> SRVLLALHDRAPQLKISDDRLTVVGEKGYSMVRASHGVRKGAWYFEITVDEMPPDTAARLGWSQPLGNLQAPLGYDKFSYSWRSKKGTKFHQSIGKHYSSGYGQGDVLGFYINLPEDISGRGSEIIFYKNGVNQGVAYKDIFEGVYFPAIS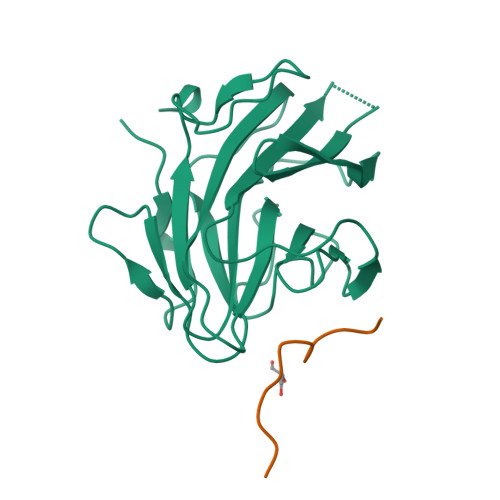LYKSCTVSINFGPCFKYPPKDLTYRPMSDMG;> EYEERESEFDIE>[2x]GSTIVGLHYKIGKKIGEGSFGVLFEGTNMINGVPVAIKFEPRKTEAPQLRDEYKTYKILNGTPNIPYAYYFGQEGLHNILVIDLLGPSLEDLFDWCGRKFSVKTVVQVAVQMITLIEDLHAHDLIYRDIKPDNFLIGRPGQPDANNIHLIDFGMAKQYRDPKTKQHIPYREKKSLSGTARYMSINTHLGREQSRRDDMEALGHVFFYFLRGHLPWQGLKAPNNKQKYEKIGE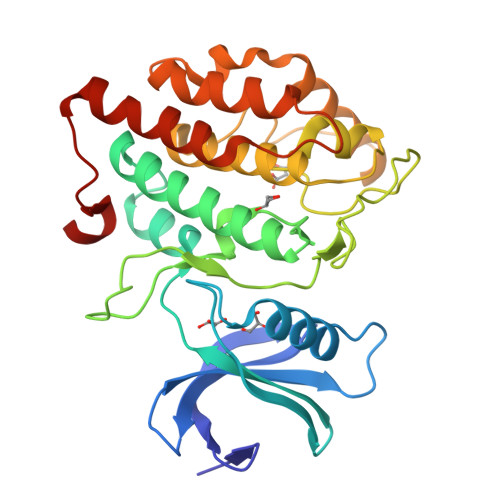KKRSTNVYDLAQGLPVQFGRYLEIVRSLSFEECPDYEGYRKLLLSVLDDLGETADGQYDWMKL The salicylate synthase MbtI from Mycobacterium tuberculosis (Mtb, the etiological agent of TB) is the first enzyme involved in the biosynthesis of mycobactins. These small-molecule siderophores are capable of chelating iron, a key cofactor involved in several mycobacterium-specific biological processes. MbtI has been structurally and biochemically characterized;2 it is essential for the survival of Mtb under iron-deficient conditions, and, as such, it has been identified as a promising therapeutic target. MbtI belongs to the group of structurally homologous Mg2+-dependent menaquinone, siderophore, and tryptophan (MST) enzymes, which transform chorismate by rearrangement, to generate precursor molecules for the respective biosynthetic pathways.

Considering the inherent difficulty in obtaining MbtI–Mg2+ cocrystals and the results of our biochemical assays, we hypothesized that we could compensate for the rather low affinity of MbtI for its cofactor by using saturating concentrations of Mg2+. Interestingly, 2.1 Å resolution data were collected from a non-isomorphous crystal grown under these conditions. In chain A, the Mg2+ interacts with the oxygen of Gly421, with four ordered water molecules, and with a sulfate anion. The coordination pattern of Mg2+ in chains B and D is analogous: the ion could be modeled as directly interacting with Glu297, Glu434, and two ordered water molecules, which in turn make H-bonds to Glu294 and Glu431. The salicylate coordinates the Mg2+ ion with its carboxylic moiety, which also forms additional H-bonds with the peptide backbone through Gly270 and Gly421 and with the side chain of Thr271. As previously noted, the bond between the carboxylic function and Gly270–Thr271 is responsible for the adoption of the closed conformation. The presence of bound salicylate in the structure is remarkable, especially considering that the natural substrate was not added to the crystallization solution. Unsurprisingly, the position that was occupied by the pyruvate is here taken by a sulfate ion, provided in the crystallization solution as the Mg2+ counterion. Observing such a conformation in this ternary complex is not surprising when high concentrations of Mg2+ are present; consistent with previous hypothesis and biochemical data, the bound Mg2+ ion stabilizes the enzyme in a close conformation, which in turn prevents the loss of salicylate from the active site.

>GHMSELSVATGAVSTASSSIPMPAGVNPADLAAELAAVVTESVDEDYLLYECDGQWVLAAGVQAMVELDSDELRVIRDGVTRRQQWSGRPGAALGEAVDRLLLETDQAFGWVAFEFGVHRYGLQQRLAPHTPLARVFSPRTRIMVSEKEIRLFDAGIRHREAIDRLLATGVREVPQSRSVDVSDDPSGFRRRVAVAVDEIAAGRYHKVILSRCVEVPFAIDFPLTYRLGRRHNTPVRSFLLQLGGIRALGYSPELVTAVRADGVVITEPLAGTRALGRGPAIDRLARDDLESNSKEIVEHAISVRSSLEEITDIAEPGSAAVIDFMTVRERGSVQHLGSTIRARLDPSSDRMAALEALFPAVTASGIPKAAGVEAIFRLDECPRGLYSGAVVMLSADGGLDAALTLRAAYQVGGRTWLRAGAGIIEESEPEREFEETCEKLSTLTPYLVARQ[4x]> QEPQPEQDPFELSGKWITSYIGSSDLEKIGENAPFQVFMRSIEFDDKESKVYLNFFSKENGICEEFSLIGTKQEGNTYDVNYAGNNKFVVSYASETALIISNINVDEEGDKTIMTGLLGKGTDIEDQDLEKFKEVTRENG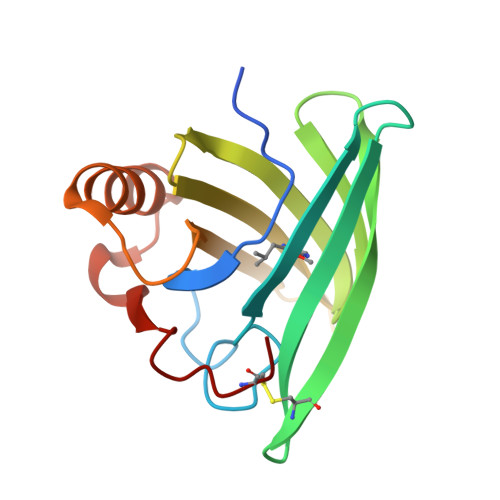IPEENIVNIIERDDCPA>[2x]GSMRDPNFQNIDKVALLGAQPLGSSHPPGDPHAVSFSLPTWASVAGNMAGEAWVRGKKKTTYPRMGFCPIVGGLTEAALIRVKRPTGVKARIFISREAAS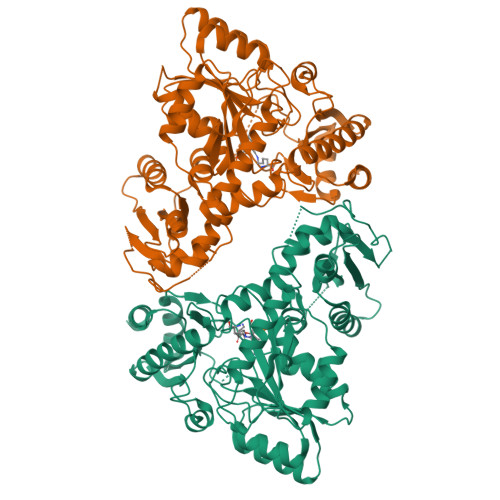RLEHTVKVKDPAAKVSVVQFELRQSNSPDLSNWARFVLVLFPESFEEDAFTFWLNHGDGISNRHAEFCNNLLDFMDSRCDEDEPDYQTCGPRSGDKPAGLPTWTNSGLEEKMVIKSVLAKCIRSENADMLPVQSDDVFLYSTGMMAIGKIARAMKDMPGDDTAVIFGWLYSGTLPLVKDSGYSKPILYGRGTEEELDKLESYLAAGGKCTVLFTEITSNPQLHSPNLVRIKNLADEYGFTVVVDDTIGTSVNLDILPYADVVTTSLTKIFNGACNAMGGSLIVNPNSRHYRRIHTYLQGHFEDLLFPADAVVLSENCIDYPERVKRCSATARAIAHFLAAHPSIDYVNYPTLVPSREEYERYRRDGEGYGYLLSIVFREPDFAVRFFDALDIWKGPSIGTNSSIALPYSVLAHWEEQDWAAEYGVPKHIVRLSVGLESEAWLRDRVTEALAKATPATLCRTTFCKSER>[4x]AKRKRIEMYTKASFKASNQKIEQIWKTQQEEIQKLNNEYSQQFMNVLQQWELDIQKFEEQGEKLSNLFRQQQKIFQQSRIVQSQRMKAIKQIHEQFIKSLEDVEKNNDNLFTGTQSELKKEMAMLQKKVMMETQQQEMANVRKS

A highly-conserved meiosis-specific structure, the chromosome axis, assembles in early meiotic prophase and provides a scaffold for the organization of chromosomes as a linear array of loops, and also orchestrates the formation of DSBs and their repair as inter-homolog crossovers. Mammals possess two such proteins, SYCP2 (1500 residues in Mus musculus) and SYCP3 (254 residues), which are both required for proper axis formation and wild-type levels of crossovers, and are known to interact with one another through their C-terminal coiled-coil domains. Mammalian SYCP3 is known to form coiled-coil homotetramers that self-associate into larger structures both in cell culture and in vitro, but how SYCP3 cooperates with SYCP2 to mediate chromosome localization and axis assembly is not known. We further show that both SYCP2/SYCP3 and ASY3/ASY4 form heterotetrameric coiled-coil complexes that self-assemble into extended filaments, paralleling our findings with Red1.

We combined the truncations on both proteins to yield a minimal construct, Mm SYCP21325-1479:SYCP3105-248, which we term SYCP2CC:SYCP3CC hereon. We found that Mm SYCP3CC also forms homotetramers in the absence of SYCP2CC (not shown), and when we determined the structure of Mm SYCP3CC by x-ray crystallography, we observed an antiparallel coiled-coil homotetramer similar in structure to H. sapiens SYCP3. As SYCP2 and SYCP3 share limited sequence homology in their coiled-coil region, we reasoned that SYCP3 homotetramers may form through promiscuous coiled-coil interactions in the absence of SYCP2. To compare the stability of Mm SYCP3CC homotetramers with Mm SYCP2CC:SYCP3CC heterotetramers, we measured their melting temperatures (Tm) using a dye-binding assay. We found that the SYCP2CC:SYCP3CC heterotetramer is more stable than SYCP3CC on its own (56.0°C Tm versus 52.5°C), supporting the idea that the heterotetrameric complex is the preferred state when both proteins are present. While the SYCP3CC homotetramer is likely not the favored state in the presence of SYCP2, its structure may nonetheless be informative as to the structure of SYCP2CC:SYCP3CC. Overall, these data show that the SYCP2CC:SYCP3CC complex forms an extended coiled-coil tetramer with an overall structure similar to that of the SYCP3 homotetramer. Using sequence alignments and the structures of H. sapiens and M. musculus SYCP3, we generated physical models for SYCP2:SYCP3 where the monomers are arranged either parallel or antiparallel, and mapped all identified crosslinks onto these models. In agreement with our SAXS data, the crosslinking data strongly support a heterotetramer model with two SYCP2 monomers arranged parallel to one another and antiparallel to two SYCP3 monomers.> ALTNLVAEPFAKLEQDFGGSIGVYAMDTGSGATVSYRAEE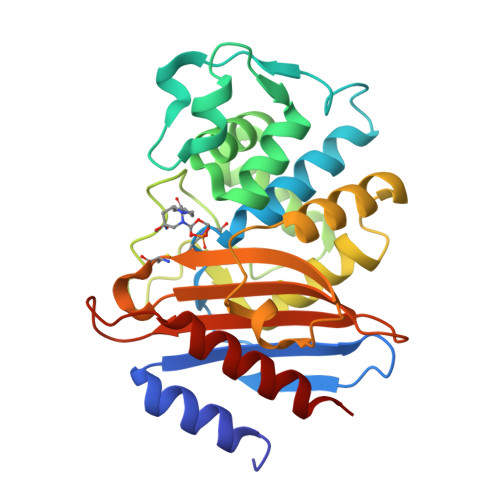RFPLCSSFKGFLAAAVLARSQQQAGLLDTPIRYGKNALVPWSPISEKYLTTGMTVAELSAAAVQYSDNAAANLLLKELGGPAGLTAFMRSIGDTTFRLDRWELELNSAIPGDARNTSSPRAVTESLQKLTLGSALAAPQRQQFVDWLKGNTTGNHRIRAAVPADWAVGDKTGTCGVYGTANDYAVVWPTGRAPIVLAVYTRAPNKDDKHSEAVIAAAARLALEGLG> GTTKHSKLLILGSGPAGYTAAVYAARANLQPVLITGMEKGGQLTTTTEVENWPGDPNDLTGPLLMERMHEHATKFETEIIFDHINKVDLQNRPF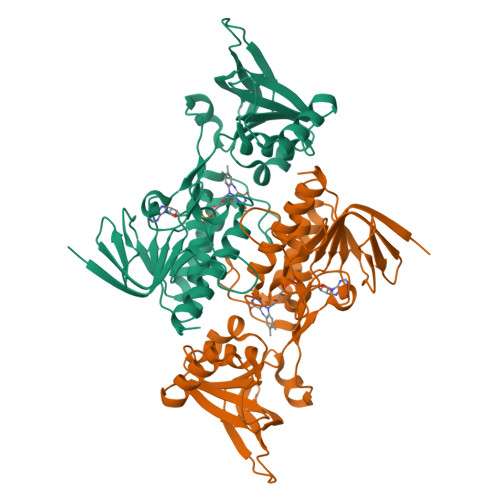RLNGDNGEYTCDALIIATGASARYLGLPSEEAFKGRGVSACATCDGFFYRNQKVAVIGGGNTAVEEALYLSNIASEVHLIHRRDGFRAEKILIKRLMDKVENGNIILHTNRTLEEVTGDQMGVTGVRLRDTQNSDNIESLDVAGLFVAIGHSPNTAIFEGQLELENGYIKVQSGIHGNATQTSIPGVFAAGDVMDHIYRQAITSAGTGCMAALDAERYLDGLADAK> GMALQLSREQG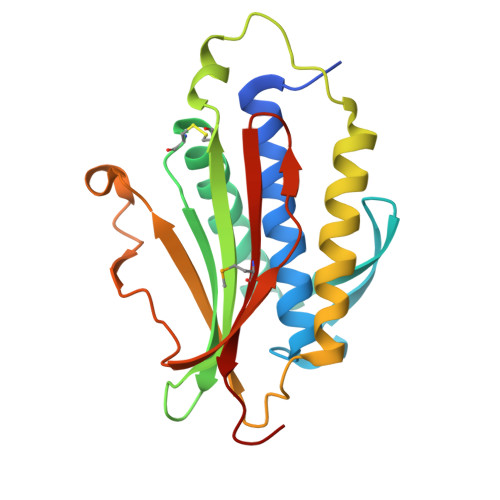ITARGSAEIVAEFFSFGINSILYQRGIYPSETFTRVQKYGLTLLVTTDLELIKYLNNVVEQLKDWLYKCSVQKLVVVISNIESGEVLERWQFDIECDKTAKDDSAPREKSQKAIQDEIRSVIRQITATVTFLPLLEVSCSFDLLIYTDKDLVVPEKWEESGPQFITNSEEVRLRSFTTTIHKVNSMVAYKIPVND>[2x]QDPIKFTTGSATPASYNQFIDALRERLTGGLI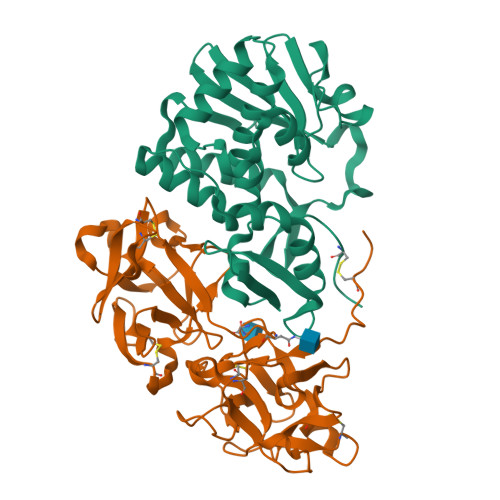YGIPVLRDPSTVEKPNQYVTVELSYSDTVSIQLGIDLTNAYVVAYRAGSESFFFRNAPASASTYLFTGTQQYSLPFDGNYDDLEKWAHQSRQRISLGLEALRQGIKFLRSGASDDEEIARTLIVIIQMVAEAARFRYVSKLVVISLSNRAAFQPDPSMLSLENTWEPLSRAVQHTVQDTFPQNVTLINVRQERVVVSSLSHPSVSALALMLFVCNPLNATQSPLLI;>VVEQSKICSSHYEPTVRIGGRDGLCVDVSDNAYNNGNPIILWKCKDQLEVNQLWTLKSDKTIRSKGKCLTTYGYAPGNYVMIYDCSSAVAEATYWDIWDNGTIINPKSGLVLSAESSSMGGTLTVQKNDYRMRQGWRTGNDTSPFVTSIAGFFKLCMEAHGNSMWLDVCDITKEEQQWAVYPDGSIRPVQNTNNCLTCEEHKQGATIVMMGCSNAWASQRWVFKSDGTIYNLYDDMVMDVKSSDPSLKQIILWPYTGNANQMWATLF[2x]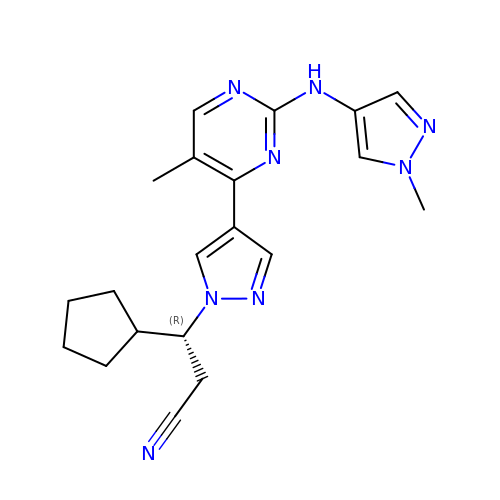(3R)-3-cyclopentyl-3-[(4M)-4-{5-methyl-2-[(1-methyl-1H-pyrazol-4-yl)amino]pyrimidin-4-yl}-1H-pyrazol-1-yl]propanenitrile | C20 H24 N8 | FEQOESZUGZISHK-GOSISDBHSA-N>[6x]MGHHHHHHMKTPPINQKSLRETESWKLLESSIIYYEGNPIGTVAAQDPELAA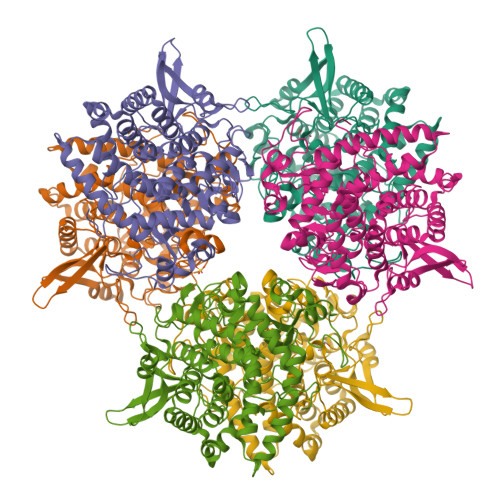LNYDQCFLRDFVPSAFVFLMDGQTDIVRNFLIETLTLQSHEKEMDCFQPGAGLMPASFKVESDGSKEYLVADFGEKAIARVPPVDSCMWWILLLRAYEKATGDLTLAREPKFQAGIKLILDLCLAHRFSMYPTMLVPDGAFMIDRRMGVYEHPLEIQVLFYAALRAARELLLPDGDGEQYLNKVHGRLGALQYHIRNYYWVDLKRLREIYRYKGNEFGKEIANKFNIFSQSIPDWVIEWLPEKGGYLAGNLGPGRMDFRFFALGNLMAILAGLASEEESQRIMNLFAHRWEDLIGYMPVKICYPALQGLEWQIVTGCDPKNIPWSYHNGGNWPVLLWLFTAAALKTGKVELAHEAIAIAEGRLSNDKFPEYYDGNNGRLIGKEARIYQTWSIAGLLVAKQFLANPDHVEFISFPDTFIGPGCSL> MGSSHHHHHHSSENLYFQSHMTLPAFKAYDIRGRVPDELNEDLARRIGVALAAQLDQGPVVLGHDVRLASPALQEALSAGLRASGRDVIDIGLCGTEEVYFQTDYLKAAGGVMVTASHNPMDYNGMKLVREQARPISSDTGLFAIRDTVAADTAAPGEPTASEQSRTDKTAYLEHLLSYVDRSTLKPLKLVVNAGNGGAGLIVDLLAPHLPFEFVRVFHEPDGNFPNGIPNPLLPENRDATAKAVKDNGADFGIAWDGDFDRCFFFDHTGRFIEGYYLVGLLAQAILAKQPGGKVVHDPRLTWNTVEQVEEAGGIPVLCKSGHAFIKEKMRSENAVYGGEMSAHHYFREFAYADSGMIPWLLIAELVSQSGRSLADLVEARMQKFPCSGEINFKVADAKASVARVMEHYASLSPELDYTDGISADFGQWRFNLRSSNTEPLLRLNVETRGDAALLETRTQEISNLLRG

The α-D-phosphohexomutases are ubiquitous enzymes found in all kingdoms of life. Among other reactions, these enzymes catalyze the reversible conversion of 1-phospho to 6-phosphohexoses, with various sugars including glucose, mannose, glucosamine, and N-acetylglucosamine. In bacteria, the enzymes phosphoglucomutase (PGM) and phosphomannomutase/phosphoglucomutase (PMM/PGM) are involved in the biosynthesis of exopolysaccharides that contribute to the pathogenicity of infections in higher organisms, including humans, animals, and plants. The reaction mechanism of the α-D-phosphohexomutases is conserved, and entails two phosphoryl transfers [Fig. 1(a)], with the initial transfer occurring from a phosphoserine residue of the enzyme to a monophosphorylated sugar to form a bisphosphorylated intermediate (e.g., glucose 1,6-bisphosphate or G16P).

The structure of apo-XcPGM was determined with both the phosphorylated (EP; active) and unphosphorylated (EdeP; inactive) states of the catalytic serine. To obtain phospho-enzyme crystals, the purified protein was phosphorylated with G16P prior to crystallization and crystals grown at 4 °C to limit spontaneous hydrolysis of the phosphoserine. Overall, the structures of EP and EdeP are very similar, with a Cα root-mean-square deviation (RMSD) between polypeptide backbones of 0.26 Å. A small shift in the backbone between these two structures is evident in loop (i) and several other regions near the site of phosphorylation [Fig. 3(a)]. In EP, one of the phosphate oxygens takes the place of the serine hydroxyl and coordinates the metal along with the aspartates in loop (ii). A structural shift of loop (i) between EP and EdeP has not been observed in other enzymes in the superfamily, although only a few have been crystallized in both states. In PC1, a distinct separation is seen between the two apo structures (triangles) and the ligand complexes (circles). This variation is the most significant in the data set, consistent with the obvious conformational change of loop (iv) upon ligand binding.>QDSTSDLIPAPPLSKVPLQQNFQDNQFQGKWYVVGLAGNAILREDKDPQKMYATIYELKEDKSYNVTSVLFRKKKCDYWIRTFVPGCQPGEFTLGNIKSYPGLTSYL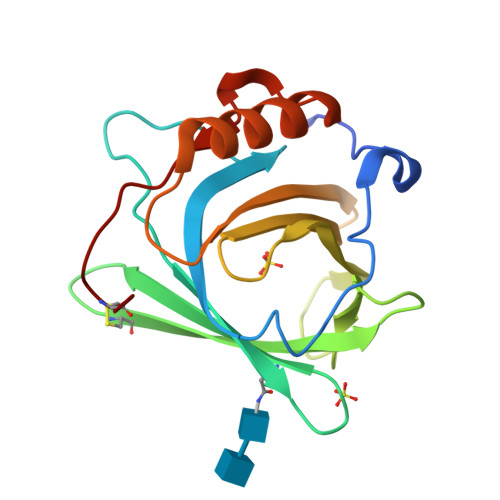VRVVSTNYNQHAMVFFKKVSQNREYFKITLYGRTKELTSELKENFIRFSKSLGLPENHIVFPVPIDQCID[2x]>HPETLVTVKDIESRLGARVGYAVLDTASGKIWESYRADERFPMMSTFKVLACGALLSRVDAGQEQLDRRIRFRQSDLVTYSPVTEKHLDDGMTLAELCEAAITMSDNTAGNLVLETLGGPEGLTAFLRTL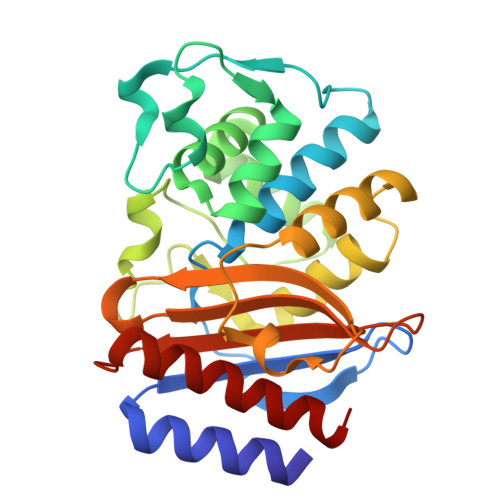GDQVTRLDRWETALNEATPGDERDTTTPAAMAATLRKLLTGDALSPASRQQLIDWMEADKVAGPLLRSALPAGWFIADKSGAGGRGSRGIVAALGPPGKPPRIVVIYLTETEATMDERNAAIAEIGAALIKHW[2x]> GUGUGCCCGGCAUGGGUGCAGUCUAUAGGGUGAGAGUCCCGAACUGUGAAGGCAGAAGUAACAGUUAGCCUAACGCAAGGGUGUCCGUGGCGACAUGGAAUCUGAAGGAAGCGGACGGCAAACCUUCGGUCUGAGGAACACGAACUUCAUAUGAGGCUAGGUAUCAAUGGAUGAGUUUGCAUAACAAAACAAAGUCCUUUCUGCCAAAGUUGGUACAGAGUAAAUGAAGCAGAUUGAUGAAGGGAAAGACUGCAUUCUUACCCGGGGAGGUCUGGAAACAGAAGUCAGCAGAAGUCAUAGUACCCUGUUCGCAGGGGAAGGACGGAACAAGUAUGGCGUUCGCGCCUAAGCUUGAACCGCCGUAUACCGAACGGUACGUACGGUGGUGUGAGAG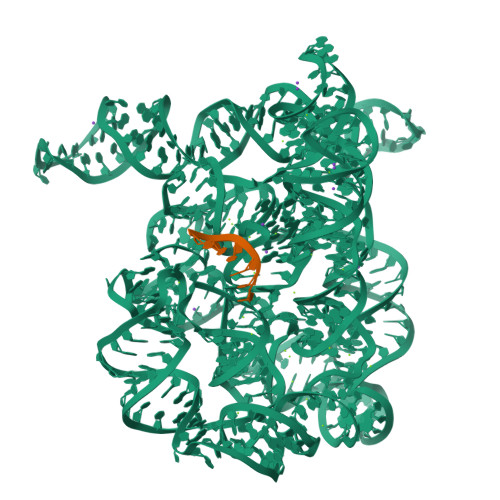GAGUUCGCUCUACUCUAU;> UUAUUA> HSAFAADPGHAGTTYIFSKGGGQITYKWPPNDRPSTRADRLAIGFSTVQKEAVLVRVDSSSGLGDYLELHIHQGKIGVKFNVGTDDIAIEESNAIINDGKYHVVRFTRSGGNATLQVDSWPVIERYPAGRQLTIFNSQATIIIGGKEQGQPFQGQLSGLYYNGLKVLNMAAENDANI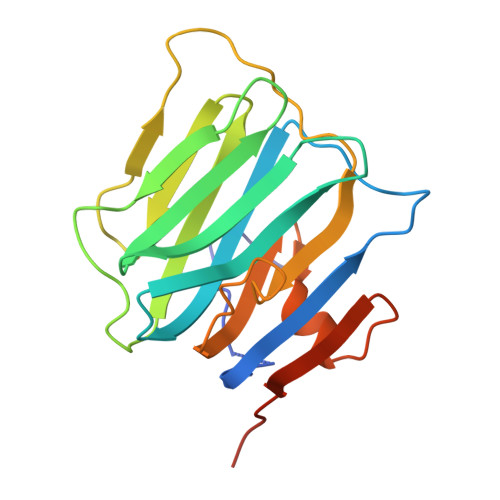AIVGNVRLVGEVPHHHHHHH> X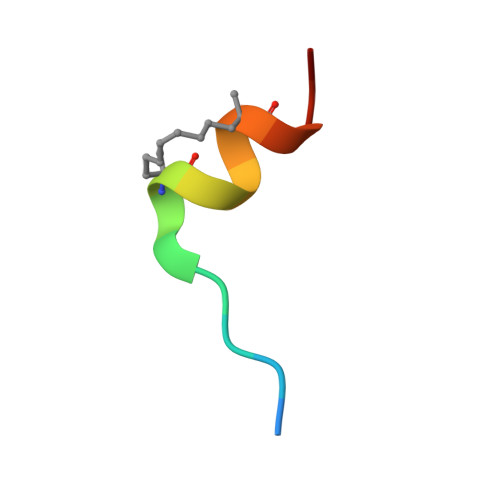KKRYSRLQLLLFRRR>[3x]MAHHHHHHMPSERTFIAVKPDGVQRNLVGEIIKRFENKGYKLVGLKLLQPTEEQAKQHYIDLASKPFYSGLVSYFSSGPIVGMVWEGLGVVKGGRVLLGATNPADSLPGTIRGD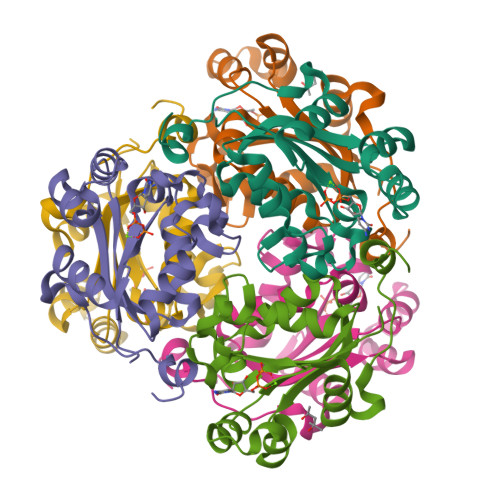FAVDVGRNVCHGSDSVESAKREIAFWFKAEELVSWTSHSVKQIYERA>[2x]MSTVPELLARQVTRAPDAVAVVDRDRVLTYRELDELAGRLSGRLIGRGVRRGDRVAVLLDRSADLVVTLLAIWKAGAAYVPVDAGYPAPRVAFMVADSGASRMVCSAATRDGVPEGIEAIVVTDEEAFEASAAGARPGDLAYVMYTSGSTGIPKGVAVPHRSVAELAGNPGWAVEPGDAVLMHAPYAFDASLFEIWVPLVSGGRVVIAEPGPVDARRLREAISSGVTRAYLTAGSFRAVAEESPESFAGLREVLTGGDVVPAHAVARVRSACPRVRIRHLYGPTETTVCATWHLLEPGDEIGPVLPIGRPLPGRRAQVLDASLRAVAPGVIGDLYLSGAGLADGYLRRAGLTAERFVADPSAPGARMYRTGDLAQWTADGALLFAGRADDQGSHHHHHH;>[2x]MTNPFDNEDGSFLVLVNGEGQHSLWPAFAEVPDGWTGVHGPASRQDCLGYVEQNWTDLRPKSLISQISD

In this work, we have sought to understand the evolutionary history of lipid II targeting glycopeptide antibiotics (GPAs), a vital class of nonribosomal peptides used in the clinic for the treatment of resistant bacterial infections and exemplified by vancomycin (Van) and teicoplanin (Tei). Since ANC1-3 domains display polydisperse elution profiles in size exclusion chromatography, we instead turned to the characterisation of an Acore construct of the Hpg accepting A1 domain from Tei biosynthesis (A1tei), which possesses a homologous pocket to ANC1. The MbtH-like domain Tcp13 also exhibits the anticipated fold, containing a 3-stranded antiparallel β-sheet and an α-helix adjoining the centre of the sheet.

To understand the effects of the evolutionary mutations seen in the binding pocket of the ANC A-domains we then mutated the residues of the substrate binding pocket of A1tei to those seen in A1ANC2 and A1ANC3. Comparison of the A1ANC2 pocket with the A1tei/ANC1 Hpg pocket revealed that the amino acid substitutions contribute both to prevent Hpg binding and opening the pocket to accept proteinogenic amino acids instead of Hpg. The substitution H237Y is key in this process, as it removes H-bonding to the 4-hydroxyl group of Hpg and narrows the pocket to exclude the planar Hpg residue. The L295V mutation then opens a cavity that allows the binding of proteinogenic amino acids with a 109° angle at the β carbon. These two key substitutions (H237Y and L295V) enabled binding of new substrates and potentiated the binding pocket for subsequent refinement and partition of substrate binding mode. Activity of ANC2int is consistent with this being an intermediate pocket, showing reduced activity that is improved through natural selection, and supports Van-type GPAs as being older than Pek-type GPAs. No substrate bound structure was obtained for A1ANC2 and ANC4, with substrates shown in stippled lines and greyed out to show an approximate position of bound substrate. The ability to interrogate the stepwise changes in the GPA NRPS via mutation of A1 provides important insights into their evolutionary process, showing that the switch from Hpg (ANC1) to Leu (ANC3) did not result in an intermediate pocket (ANC2) capable of activating both residues. Instead, this was a direct selectivity switch that was subsequently refined to provide the modern Van-type GPA A1-domains.>MVQPSLPQDDTPDQQEQRNRAIAQQREAYQYSETAGILLIKTLPQSEMFSLKYLIERDKGLVSLIANTLASNIENIFDPFDKLEDFEEMFPLLPKPLVMNTFRNDRVFARQRIAGPNPMVIERVVDKLPDNFPVTDAMFQKIMFTKKTLAEAIAQGKLFITNYKGLAELSPGRYEYQKNGTLVQKTKTIAAPLVLYAWKPEGFGDYRGSLAPIAIQINQQPDPITNPIYTPRDGKHWFIAKIFAQMADGNCHEAISHLARTHLILEPFVLATANELAPNHPLSVLLKPHFQFTLAINELAREQVISAGGYADDLLAGTLEASIAVIKAAIKEYMDNFTEFALPRELARRGVGIGDVDQRGENFLPDYPYRDDAMLLWNAIEVYVRDYLSLYYQSPVQIRQDTELQNWVRRLVSPEGGRVTGLVSNGELNTIEALVAIATQVIFVSGPQHAAVNYPQYDYMAFIPNMPLATYATPPNKESNISEATILNILPPQKLAARQLELMRTLCVFYPNRLGYPDTEFVDVRAQQVLHQFQERLQEIEQRIVLCNEKRLEPYTYLLPSNVPNSTSI[2x]

Lipoxygenases (LOX) are key enzymes in the initial step of lipid-mediator biosynthesis. They catalyze a regio- and stereo specific dioxygenation of polyunsaturated fatty acids to yield fatty acid hydroperoxides, which can be further metabolized to a variety of signaling molecules with diverse biological functions. CspLOX2 is the LOX with the highest relative amount of bis-allylic product reported so far, hence it is a suitable candidate to study the molecular basis of the dioxygen positioning at the bis-allylic position. We demonstrate the importance of an active site clamp around the pentadiene system, which fixes the pentadiene during the reaction resulting in 11-HPODE formation.

A key residue that is located opposite of the iron ion and hence likely restricts the space in the kink region is the highly conserved Leu304. Exchange of this residue for a less bulky valine reduced the relative amount of 11-HPODE to 30% compared to 74% produced by CspLOX2 wt (wild type). In case of 13-HPODE, Leu304 and Leu502 are rather facing the side of 13S-HPODE formation, while Leu506 faces the side for 13R-HPODE formation. Consequently, if more space is created by decreasing the size of one amino acid, dioxygenation at the nearest position on the linoleic acid substrate is preferred over other possible dioxygenation sites. We found that the ability to produce 11-HPODE was diminished by widening the active site clamp in CspLOX2, while the production of 11-HPODE could be induced in its isoenzyme CspLOX1 by reducing the space in the channel.[5-(4-aminophenyl)furan-2-yl]methanol | 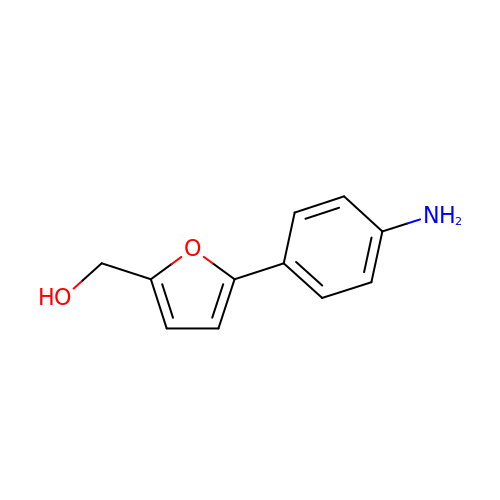C11 H11 N O2 | PGRYIWSQXZECGD-UHFFFAOYSA-N>KETAAAKFERQHMDSSTSAASSSNYCNQMMKSRNLTKDRCKPVNTFVHESLADVQAVCSQKNVACKDGQTNCYQSYSTMSI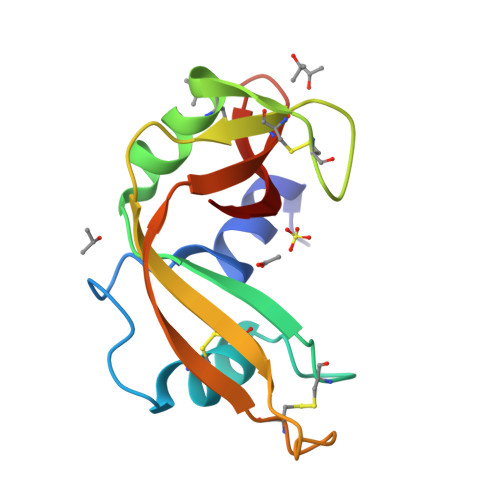TDCRETGSSKYPNCAYKTTQANKHIIVACEGNPYVPVHFDASV[2x]> MKKVKLIGTLDYGKYRYPKNHPLKIPRVSLLLRFKDAMNLIDEKELIK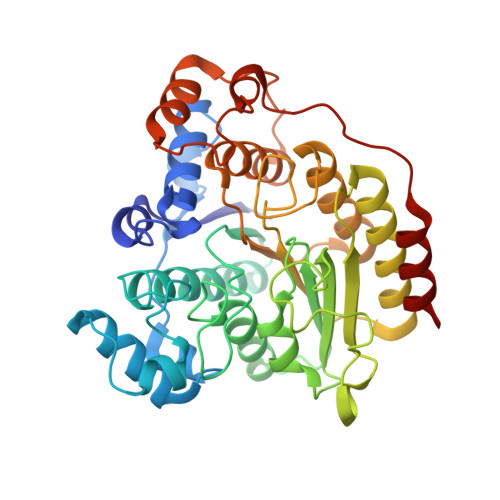SRPATKEELLLFHTEDYINTLMEAERCQCVPKGAREKYNIGGYENPVSYAMFTGSSLATGSTVQAIEEFLKGNVAFNPAGGMHHAFKSRANGFCYINNPAVGIEYLRKKGFKRILYIDLDAHHCDGVQEAFYDTDQVFVLSLHQSPEYAFPFEKGFLEEIGEGKGKGYNLNIPLPKGLNDNEFLFALEKSLEIVKEVFEPEVYLLQLGTDPLLEDYLSKFNLSNVAFLKAFNIVREVFGEGVYLGGGGYHPYALARAWTLIWCELSGREVPEKLNNKAKELLKSIDFEEFDDEVDRSYMLETLKDPWRGGEVRKEVKDTLEKAKASS>X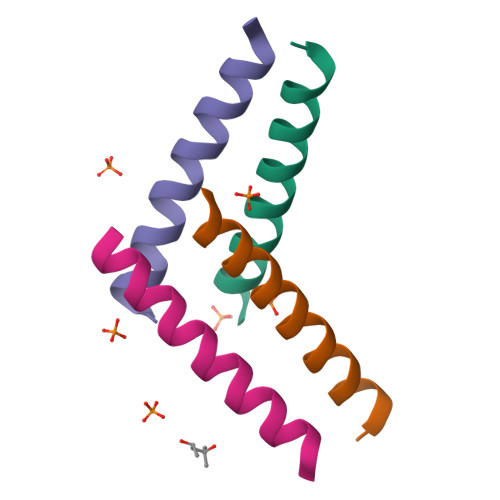SKLLELLRKLLEALHKAIELLEKWGX[4x]>MALSAEGSSGGSRGGSPKAEAASVPSWPQILGRLTDNRDLARGQAAWAMDQIMTGNARPAQIAAFAVAMTMKAPTADEVGELAGVMLSHAHPLPADTVPDDAVDVVGTGGDGVNTVNLSTMAAIVVAAAGVPVVKHGNRAASSLSG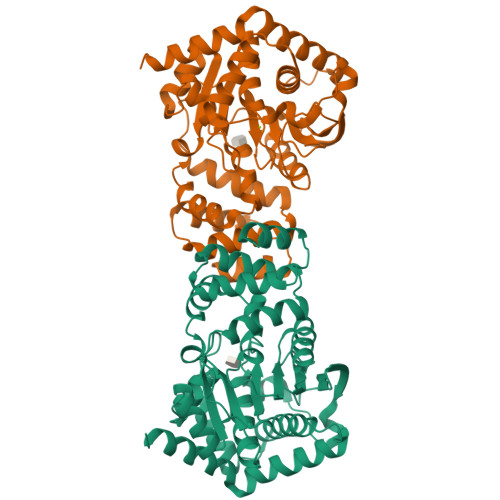GADTLEALGVRIDLGPDLVARSLAEVGIGFCFAPRFHPSYRHAAAVLREIGVPTVFNLLGPLTNPARPRAGLIGCAFADLAEVMAGVFAARRSSVLVVHGDDGLDELTTTTTSTIWRVAAGSVDKLTFDPAGFGFARAQLDQLAGGDAQANAAAVRAVLGGARGPVRDAVVLNAAGAIVAHAGLSSRAEWLPAWEEGLRRASAAIDTGAAEQLLARWVRFGRQILEHHHHHH[2x]>[2x]MAVFEQNKRPKIALVGSGMIGGTMAFLCSLKELGDVVLFDVVPNMPMGKAMDLCHNSSVVDNGITVYGSNSYECLTNADVVIITAGITKIPGKSDKEWSRMDLLPVNIKIMREVGGAIKKYCPNAFIINITNPLDVMVAAVQEAANVPKHMICGMAGMLDSSRLRRMIADCLH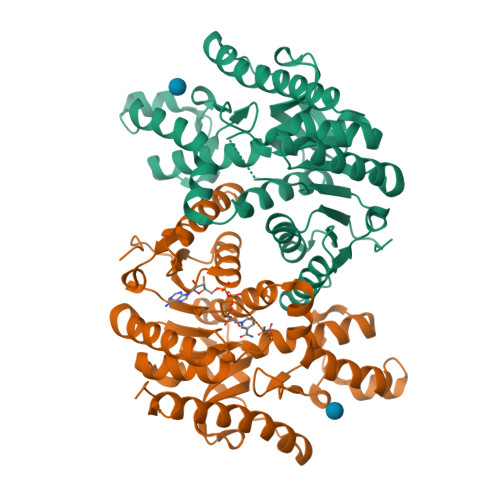VSPHDVQGMVIGVHGDNMLPLMRYITINGIPIQEFINKGLINKEDINNIYNKTKQAGGDIVRLLGQGSAYYAPGTSAILMAESYLKDKKRLFVSSCYLNGQYNVNNHYLGVPCIIGGKGIEQIIELDLNQEEKKLLQGSIDEVLEMQKAIAALDAGKLEHHHHHH> EKRKAAAAILSLGNVLNYLDRYTVAGVLLDIQQHFGVKDRGAGLLQSVFICSFMVAAPIFGYLGDRFNRKVILSCGIFFWSAVTFSSSFIPQQYFWLLVLSRGLVGIGEASYSTIAPTIIGDLFTKNTRTLMLSVFYFAIPLGSGLGYITGSSVKQAAGDWHWALRVSPVLGMITGTLILILVPATKRGHADQLGDQLKARTSWLRDMKALIRN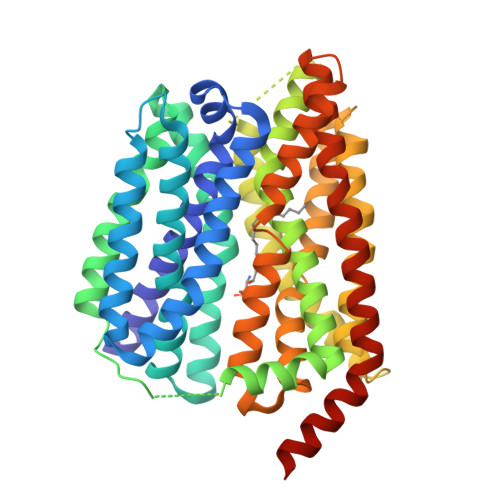RSYVFSSLATSAVSFATGALGMWIPLYLHRAQVVQKTAETCNSPPCGAKDSLIFGAITCFTGFLGVVTGAGATRWCRLKTQRADPLVCAVGMLGSAIFICLIFVAAKSSIVGAYICIFVGETLLFSNWAITADILMYVVIPTRRATAVALQSFTSHLLGDAGSPYLIGFISDLIRQSTKDSPLWEFLSLGYALMLCPFVVVLGGMFFLATALFFVSDRARAEQQVNQLAMPPASVKV>[10x]SLINTKIKPFKNQAFKNGEFIEVTEKDTEGRWSVFFFYPADFTFVCPTELGDVADHYEELQKLG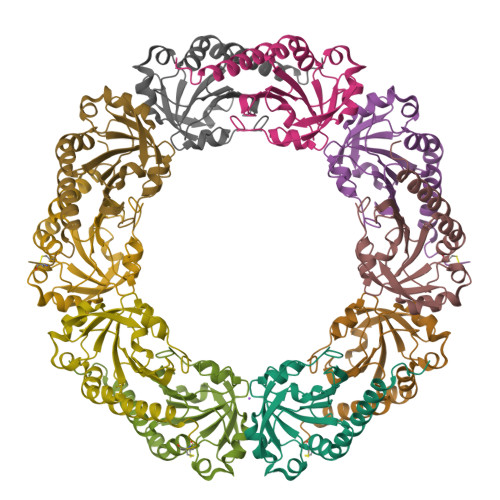VDVYSVSTDTHFVHKAWHSSSETIAKIKYAMIGDPTGALTRNFDNMREDEGLADRATFVVDPQGIIQAIEVTAEGIGRDASDLLRKIKAAQYVAAHPGEVCPAKWKEGEATLAPSLDLVGKI> ADSTITI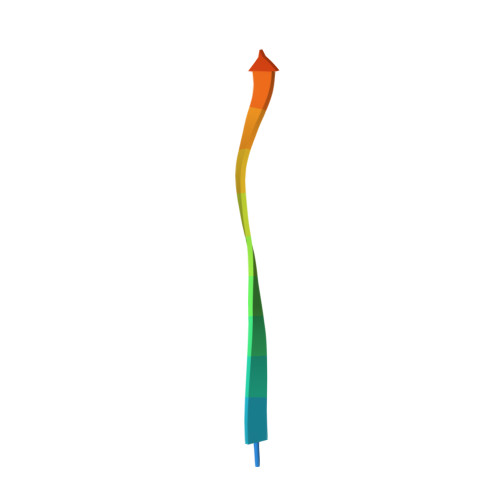RGYVRDNR>[4x]GSHMSVVISDAWRQRFGGTARLYGEKALQLFADAHICVVGIGGVGSWAAEALARTGIGAITLIDMDDVCVTNTNRQIHALRDNVGLAKAEVMAERIRQINPECRVTVVDDFVTPDNVAQYMSVGYSYVIDAIDSVRPKAALIAYCRRNKIPLVTTGGAGGQIDPTQIQVTDLAKT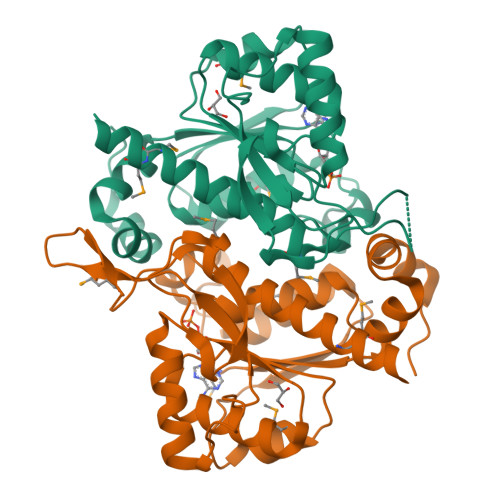IQDPLAAKLRERLKSDFGVVKNSKGKLGVDCVFSTEALVYPQSDGTVCAMKATAEGPKRMDCASGFGAATMVTATFGFVAVSHALKKMMAKAARQG> EELFNALPQPLQQLSLALAGEIPLTDHIFEQAASTWHVQPRSLTYKLLDHIPFSTPVVVPPSIYHSLDWSKCFAVNQDRVERVPTIDDPDDVYVPNSDIGPLLTSLHTIPDYGFLHPAIENDATTLRAERARCASTFYKIASSQARQVKLDPIRMLGFLLLVQARPRVPSGLVTDQPTRRDPTQSPALHAIWQVMQYYKVAGVYYAPALVVPSGAIWWIPPPGKRNVVSVQYLLTDLINLAILAHMTDMSPTLELTGVLMYLRAASSHSHAYTLLQMKSVFPALSLRSMYRNKGFGGKAPAIEWTEPRSKYKFRWTGVTQLHDGLRPRSPSMDVPTLEVLTKYELVDIGHIIIRERNAHPRHNHDSVRFVRDVMALTSGMYLVRQPTMSVLREYSQVPDIKDPIPPSAWTGPIGNVRYLLPSVQGPARHLYDTWRAAARQIAQDPQWHDPLNQAIMRAQYVTARGGSSASLKFALKVTGIVLPEYDDSKVKKSSKIYQAAQIARIAFMLLIAAIHAEVTMGIRNQVQRRARSIMPLNVIQQAISAPHTLVANYINKHMNLSTTSGSVVTDKVIPLILYASTPPNTVVNVDIKACDASITYNYFLSVICGAMHEGFEVGNADAAFMGVPSTIVSDRRSSVAPYSRPISGLQTMVQHLADLYAAGFRYSVSDAFSSGNKFSFPTSTFPSGSTATSTEHTANNSTMMEYFLNVHAPSHVKSASLKRILTDMTIQRNYVCQGDDGILLLPHEAASKISADDMNELLTCLRDYGQLFGWNYDIDWSDTAEYLKLYALMGCRIPNTSRHPPVGKEYAAPQTDEIWPSLIDIVIGHHLNGVTDVLNWREWLRFSWAFACYSSRGGYTNPKGQSFSAQYPWWTFVYLGIPPILLPGQTPFIHSCYMPPGDQGMFSILNGWRDWLISHASTTLPPLRHNHPVWGLSDVPSLLSQFGVYAGYHAAQHYRRPKPAPETASSDSINQITSDLTEYLFYDSALKARVMKGRYNWERLSSSLSLNVGSRVPSLFDVPGKWVAAGRDAEKPPPSSVEDMFTSLNRCIRRPTHSFSRLLELYLRVHVTLGESIPLAIDPDVPQVAGADPANDDHWFKYTCLGDIPSATRNYFGESLFVGRVVSGLDVEAVDATLLRLKILGAPPEAFIAVLNGIGMSDSEAHQIAGRISLANAQLVQIARVVHLSIPSSWMTLNTGPYIHHHAYDFKPGITQPSAKSRDKSIWMSPILKLLCTSYAMTVAGPVRTSIVTEIDGSAAALSGNLRVWMRDV;> MITIVVIPTAHFSWTDTNFLNSVDYRLTSQPKIRDRFAVYAPGWLRRQLDEFSASLTASELLQALQTIPIPVKARCLLLPKPKRFAQWLLDVPSANIWHIPVTTLRATVASKHPSSDVYNYIPDHVPPSAEFDTVTRRVAAGRDIYVRSTKVLGAPLCLAAPAKYYAGYLSTHQLDGVYPDNWAPDNFHKREFCLTILPSLLGPRTFLLDVDADRDASYPLSVLWPQLRVLALKSRLLLPPVALLRRVVDPGLKPTWSADSDAAFRALRLSRPSSASKPTGFDFSALPVVDIICLFESEPDDHGRVAPGTRLTIHSVPTDLLTSLSIQEGVRYPLRQESGMFVPWVLLALLMSDDVTISGTR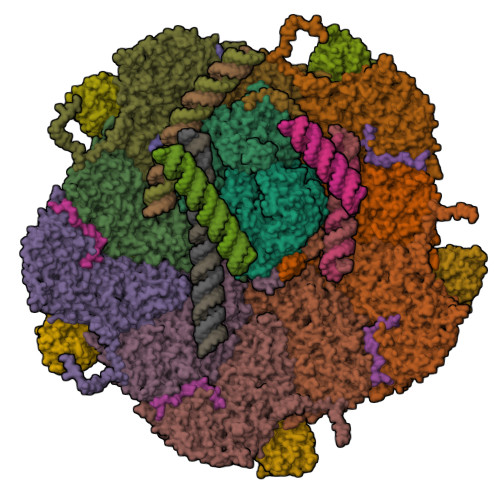RSVKLETAHASARPFVHITVERCASARVVDVRGSPAMYANAVCLTLPKGSYKSTIIDTLPAMFSDLSILEQAAVIDSDALGDSLRPSFETQFLERLENLDPKLLDRAVASILSPASDTSDDAVTTVLDVFNALYREVMTPAQRSRLPLLTQQGRVLAFAHSDYELLSANIPIQVVRGSIPIDHVVNLLARRNRVGGTALQVLLDYCYRTQASPLAPTPAGRLYKQLFGPWLMVPRLSDPLIKLRLVASAPAKVLRAAGWTIDGDPPLEVSCLCAYVTDRAMAAALIERRLDSRALVNVGGDQLMFVEYAPPLPLVSIPRTFLLPVTYVVHWVSPQRVLLNGGNVSFTSGLEWTFDD;>DIITRPTSDSIAAVANATKPAAVVSDPQSMKVTPIVNPSSYVCNVCNARFSTMSALSEHLRSDHRDDASTLLATPMINNAIRSFLTAWDGIRILSPDVSSKHLSAYLDSAVANGPELIVEDTGLCTSFMLLDNIPSAHLTKELIGFTWFMQMYQMTPPLPEGAVNRIVCMTNWASLGDEGRGLEVRLPPPTDSSVHAYKTVLSRGYIDNAQFNPLALRSNVLLMLLQFTLSNLKINKSSTFTSDVTTITSGRMIRAFEGRPELLALAYPGRAVLPTQTKNAQFLSTAIADRIGRLDRANLIGGEVSAMVECMELCDALTLHIRETYVMLLRSMHQDPTQIVQIVNECANNLLNSTIPISLRPTILCPWFASSEDLRLQQVMHLVNISSNTAAALPLVEALSTLLRSVTPLVLDPTVLTNAITTISESTTQTISPISEILRLLQPMGNDYAAFWKCIASWAYNGLVTTVLSEDAFPDSSQSITHLPSMWKCLFLTLAGPMTSDPHSPVKVFMALANLLAQPEPIAIGVPGMHQTTPASQFSHPGVWPPGFLNPQLINPQQAPLLRAFAEHIRANWPQPSEFGYGSTLQGSANLFIPPNRMVYPWPNQPLPRLTVAPTYDSAMSNWISTTIAFFIRVVNSVNMTATVNDLTRRTMTGVMTAMRQVKTMTPFYIQHMCPTELSVLASVTVTPPFQVPFTRLVQNDVITNVLVARVDPAQRGDAAVDIRATHATFAAALPVDPAAIVVAMLCGQTETNLIPSHHYGKAFAPLFASNAMFTRNQRAVITREAFVCARSAVAQCQDAGFLVPRPLDALRQFDVTSAAAAEIMHAVNDAFKTAFDLDGALLDGLALYGDPRIADLSAAYLQYGGNVVREHVPPGPSHIHRTLQQVESTFMAEMNLFNVARGNLYLVQTATNGNWSPMAPVAAPPFVRGGPNVRVVGRFGTIVPRPDGLEPQLIDDGNVPRDIAGDWVYPSDVLQVSVAVFCDYVWPMVKAGRTRVLVELGHYVYTLHYYDPQISLDEAPILEEWLSKINPAGIPPVPFCIPIPQVYPCITARRVHYAFTSENNNDSLFSTNAASIDTAFGENAAVSPLRWPGLVDPNYRVGTNDLPNRITLYNSLYRYNFTYPTLDGIMYVRSAT[10x];>[5x]TASPADTNVVPAKDAPTTNSPPSTTSPNQAAADANQQQAGIVSSQSGPNAVGDSAPSTSVNNDGDIITRPTSDSIAAVANATKPAAVVSDPQSM;>AQRQFFGLTYNFYGQPAPLFDLNDLQELAGCYARPWTSRFSHLAISTGSLPVWSARYPSVASRNIIVNTLLGAHLNPFAGGQVTSHQGITWRDPVLSSLAPVPAIQPPPVWAVAENVPLDSNNYPTYVLNLSSMWPINQDVHIMTMWALSDQGPIYHLEVPVDPMPAATTAALMAYIGVPIAHLAQTAYRFAGQLPQSPDSTMVSTIRWLSAIWFGSLTGRLNRSRTCNGFYFEFAKPALNPDQAVLKWNDGARAAPPAAAQSSYMRCISPHWQHQIVEVAGALMSQSVTAVTGLPALIDEATLPAWSQGVANLTGNGQGVVPCLDYNPVPMAAARHLQWRQDGLITAAQEAQLNNDYTAYALTIERHLTAMLVANPIAAGRMPIQPFNAADFGQAGQTAAAVALAQAMFV[10x];>AAVFGIQLVPKLNTSTTRRTFLPLRFDLLLDRLQSTNLHGVLYRALDFNPVDRSATVIQTYPPLNAWSPHPAFIENPLDYRDWTEFIHDRALAFVGVLTQRYPLTQNAQRYTNPLVLGAAFGDFLNARSIDIFLDRLFYGPTQESPITSITKFPYQWTIDFNVTADSVRTPAGCKYITLYGYDPSRPSTPATYGKHRPTYATVFYYSTLPARSRLLANLAAGPTVLEHFDSPTYGPHLLLPQTGDVLGYSSSLISQAALLMVESVMDALRDNANASASTAVTRLDQSYHPVTSFDPSTFNTLLQRATNLALLAVQGVQSESAIPAIPTMSDVRSFVARLMAEGDPQQWFPYRVDQILYWPESPFVPPIGPFYAPFRPVNFPFTTGSYTVVPDASRPLRLLPQYRNATITVQQADDAYEDTALSPLITTHGFCVTGGVSTSIYDISGDPTAYPPAQLVDTPNDYFDRERMARRDLFRRLRAPADRSAIKDRAVFDFLASLVNPTTANPVLDTSFSMAYLGASSAHANADEPVILADIRSGSIPGLPIPRRIVQFGYDVVHGSLLDLSRAVPTGTFGLVYADLDQVEDAGTDMPAANRAAIAMLGTALQMTTAGGVSVLKVNFPTRAFWTQVFNLYATHATTLHLVKPTIVNSSEVFLVFGGRQSNGALRSTTALQRALLSLYARNAAIDRAVTHIPFFGVPDDGTSDLGIDAVRLFDPMFSDAVANLPSNALASLVSRVVPSSIMFTRVPSNGPVSTTIYGKRTFLSNRRRARLRDVPMLITTTLVHQRRFTTPPTFTLFSSEAVPVTTLVAAGYNSFISEQTRNPNLAHLLDLGTGPECRILSLIPPTLQVTMSDARPCAELMASFDPALTAYVQGDYSTAAFWNGIRCDSATAIFTLGAAAAAAGTDLIAFVQQLIPRIVAAGGTRMWLQLNTPLYEVSSLPDLIDIDLRDRVYRFNGGERVEPYADPVPLQQAIAALLPAAALSWHTLSPTCDWLPYIIGVGSPLNLSDINTAISYSRLTPILHIDTTTPPLRVNPVPTPLNQQCAIRITSLDPAAVLSVQHNGVEVIGGTPGNVISVAGAAALQYILANQEFLLQFTPTLPGIFDVFLTTLGQPPVPRGSFTITPPPTTVVLNMPPPGQLDFTDVGNDARITCDPYYQLAVCIFKDGQYVRVNPEKASVVTNAPNRDLHFVLDLADNHVLLYLCDVTPSGLGDRIAFPIVDIYRIAFPRNTPVRASLPYTGGGAHLTSGGNPFMSLTTPPAVLPAGVALAALSTSVATQYPTYTLPAGVYEYVI[5x]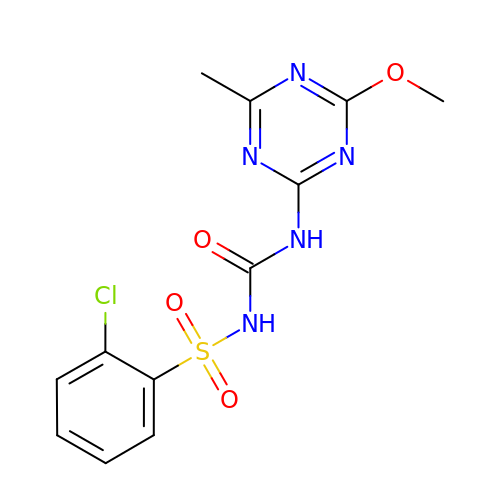1-(2-CHLOROPHENYLSULFONYL)-3-(4-METHOXY-6-METHYL-L,3,5-TRIAZIN-2-YL)UREA | C12 H12 Cl N5 O4 S | VJYIFXVZLXQVHO-UHFFFAOYSA-N> MKNVGFIGWRGMVGSVLMDRMSQENDFENLNPVFFTTSQAGQKAPVFGGKDAGDLKSAFDIEELKKLDIIVTCQGGDYTNEVYPKLKATGWDGYWVDAASA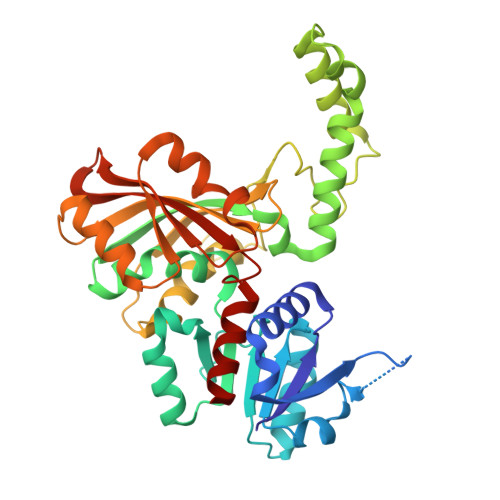LLMKDDAIIVLDPVNQHVISEGLKKGIKTFVGGNCTVSLMLMAIGGLFEKDLVEWISVATYQAASGAGAKNMRELLSQMGLLEQAVSSELKDPASSILDIERKVTAKMRADNFPTDNFGAALGGSLIPWIDKLLPETGQTKEEWKGYAETNKILGLSDNPIPVDGLCVRIGALRCHSQAFTIKLKKDLPLEEIEQIIASHNEWVKVIPNDKEITLRELTPAKVTGTLSVPVGRLRKLAMGPEYLAAFTVGDQLLWGAAEPVRRILKQLVA>MVLIFHGKPVHGAIFDMDGTMFDTERLRFQTLQQASQELIGQEFSHEYLMQCLGLSATTAEKLAQRLYGVDVPYKEIRKRADEMELEHIRKHGVPIKKGLVQVLERLRKSGLRMAVATSSRRAIAEEYLINANVYKFFDVITCGDEVEQGKPHPEIFLKAASQLHLDANQCLMFEDSENGLTSAHTSKGLTILLKDIKEPNDEMLEKAHFYYDQMYDFLTDLDQFIPVMDMPEMQEPFPQSLNQLTVGIHGFGAIGGGYIAQILSHWDGYTKPKRIIASTRNSLFREAVNAFGTYSIRYGQFSYDERIENMSIVDSDNEQQMLEMYTHSSLIALCLPEQAIESESKIIAKGLYARFNSQLETCIEPLTFLIILAKVGAKYLVMKHLKEALLELTNDEDVTEHILKEHYFCDTVVNRMVSKLSNQNLYRQLRIKHNFLEQHLEDVEQEDQIEIEDCNKLTPDQLNQASIYVDNMRRNFQPGHILQSMDLILFHSETDMPIYVEKGSPLLEKLRQVVLVDQITDIQLIKNRLWNGVHAMLAWYASLMGYESIGVAMGDHLVKAFAENLIAEVKQGLAIVLPNYAKDLDRMSQSFLDSCEYAFKD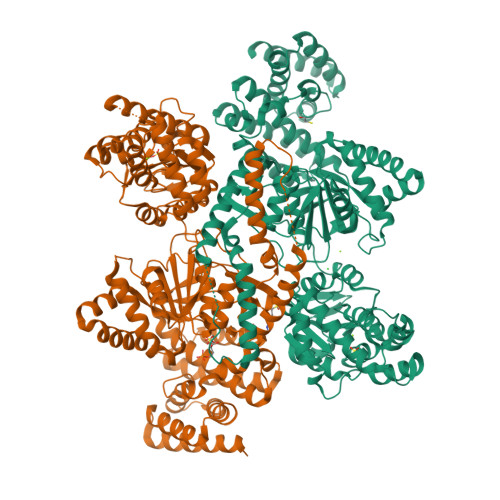PCQRVARDPLRKLNHNERVMASIAVNIRHDLPYKNLLKGAALGYAYAIQFLEIEETKAVEHLQQQIQNLDLSTAQRRQLEAELVQLIQYLFSEQGKQPLDIKSNNTKTTSTQYVAAALEHHHHHH[2x]> GQVAPNVWSKYFNIPNPGLRAYFSNVVSGQPEVYRTPFYKGMSLESICDEWYKKLVSIDTQWPTLMEFEDDLRKKVGPMSVMLPLKERMSDIDSYYDSISKDQVPFDTKAISAAKSEWKGVSRLRLRSEVNTVAVMKKSTNSGSPYFSKRKAVVSKTIPCDVYMDGRYCVMRQNGREWSGAAVLGWRGQEGGPKPTDVKQRVVWMFPFAVNIRELQVYQPLILTFQRLGLVPAWVSMEAVDRRITKMFDTKGPRDVVVCTDFSKFDQHFNPTCQSVAKELLADLLTGQEAVDWLERVFPIKYAIPLAYNWGEIRYGIHGMGSGSGGTNADETLVHRVLQHEAAISHHTTLNPNSQCLGDDGVLTYPGISAEDVMQSYSRHGLDMNLEKQYVSKQDCTYLRRWHHTDYRVDGMCVGVYSTMRALGRLAMQERYYDPDVWGEKMVTLRYLSIIENVKYHPLKEEFLDFCIKGDKTRLGLGIPGFLDNIAGEAQKAIDMMPDFLGYTKSLQYDGDLRRNAAAGIENWWV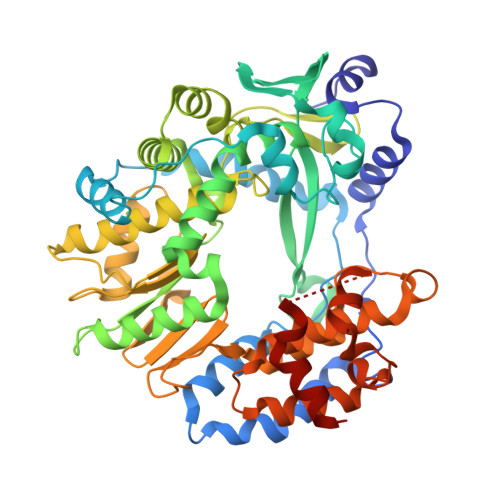VQALKSRR> TVGAVALDLDGNLAAATSTGGMTNKLPYQVGPTPLVGAGCYANNASVAVSCTGTGEVFIRALAAYDIAALMDYGGLSLAEACERVVMEKLPALGGSGGLIAIDHEGNVALPFNTEGMY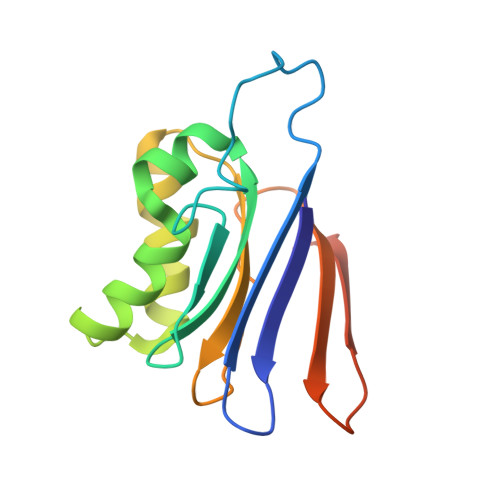RAWGYAGDTPTTGIYREKGDTVATQ>[3x]QKPNIILIVADDLGYADVGFNGSKDIITPNI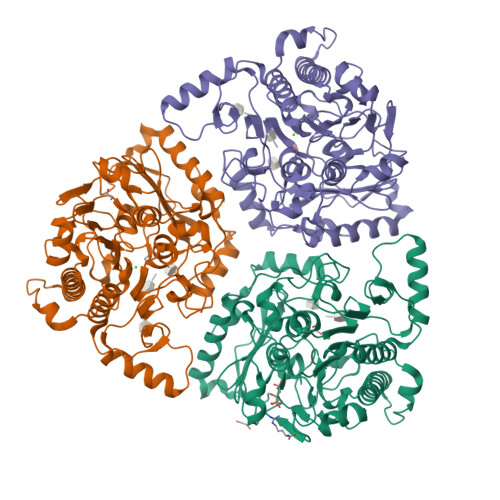DDLAKSGTSFSDAYVAHPFSGPSRAALMTGRYPHKIGSQFNLPTRGSNVGVPTDAKFISKLLNENNYFTGALGKWHMGDTPQHHPNKRGFDEYYGFLGGGHNYFPDQYQPQYKKQKAQGLKNIFEYITPLEHNGKEVKETQYITDALSREAVNFVDKAVNKKHPFFLYLAYNAPHTPLQAKDEDMAMFPNIKNKDRKTYAGMVYAVDRGVGKLVEALKKNNQYDNTLIVFMSDNGGKLSKGANNFPLKAGKGSTQEGGFRVPMLFHWPKHVPAGKRFSHPVSALDLYPTFAALAGAKVEENQHLDGTNMWPAFIKNENPHKDEPIYALRHRKGYSDAAIRMNQWKALKVNQQPWQLFNIENDISEKHDVSKSNKALLTDMVREMEKWSWDNQQPSWFHETTEGVNWRLDAMPRFDKTFKT>[2x]SNARTTTYDVFLSFRGEDTRYNFTDHLYSALGRRGIRTFRDDRLRRGEAIAPELLKAIEESRSSVIVFSENYAHSRWC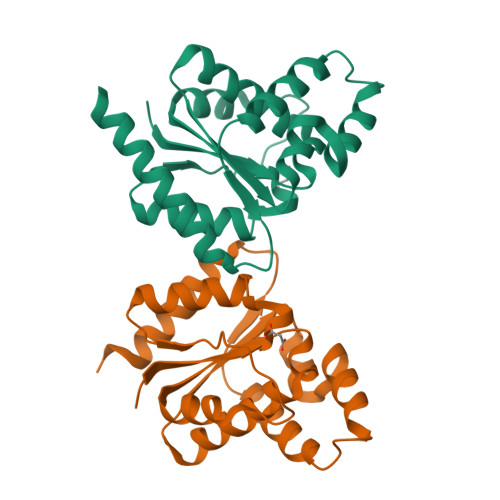LDELVKIMECQKDLGHAVFPIFYHVDPSHVRKQEGSFGEAFAGYEENWKDKIPRWRTALTEAANLSGWHLLDDRYESNQIKEITNSIFRQLKCKRLDVG> SNIVTTIYVKGDPAKNKLLDCPFCHRVLLAYEAKKLPYKMEYIDFDNKPAWLLEASGGKVPVIKEGPDAPYMPDSDVIVVHLEKQHPEPSLQSSVPAEIGAKLFPNFRAILIGPAAEVADKVAALEEQLAGMDDYLRQHEAQGPLFGGQHLNGTDCSLAPKLYHA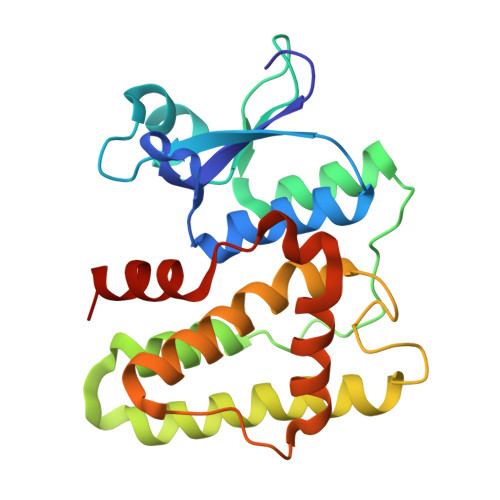VVALKHFKGWELPARFTALHKYLAALKALPEWQHVDYGTEAIIAGWERHIKH> MKKIAVLTSGGDSPGMNAAVRAVVRTAIYNEIEVYGVYHGYQGLLNDDIHKLELGSVGDTIQRGGTFLYSARCPEFKEQEVRKVAIENLRKRGIEGLVVIGGDGSYRGAQRISEECKEIQTIGIPGTIDNDINGTDFTIGFDTALNTIIGLVDKIRDTASSHARTFIIEAMGRDCGDLALWAGLSVGA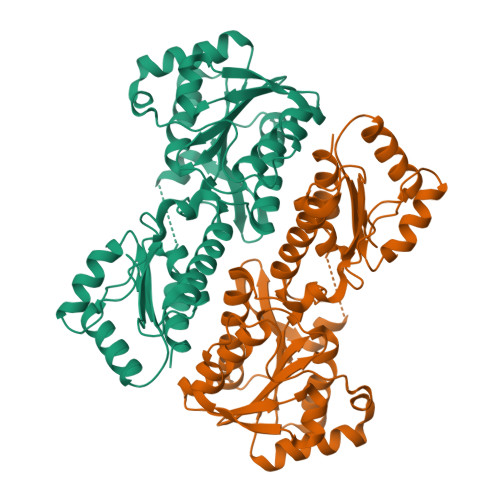ETIVVPEVKTDIKEIADKIEQGIKRGKKHSIVLVAEGCMTAQDCQKELSQYINVDNRVSVLGHVQRGGSPTGADRVLASRLGGYAVDLLMQGETAKGVGIKNNKIVATSFDEIFDGKDHKFDYSLYELANKLSI> GGTAYWKNPDQFTAFNTGLHALLREKSYNFFLLGEPRADIYGDNPIGGEASQGMERLPFNTINKENVGISNYGDMYKIINQINQMIAKTTETTILTEATQNYYLGEAYGMRAYLYFHLLRSWGDVVLYLDY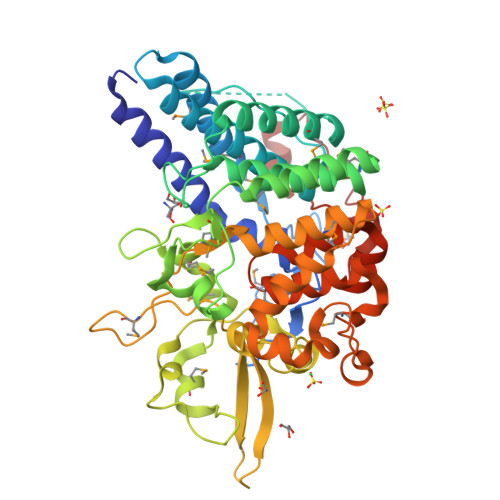TEGQNLDLSNITKGVSPATEVMEQIKKDIQASENAFGSDYSFKLGRHFWSAAATQMLKGEAYLWSGRQMNGGNSDYTIAKNAFENVKKADVGLVTSSFKDIFSFENKKNKEMIFTIHNGKDEYEMWGGYYRMRLIPAQDKMVKIYCDENGNSFVGTPDAQLNGLTQLQVRREFYFKGFRNNDTRWTTSLKAVYKKDAQGVVSYFGPITYKFQGTMLEGGSTRSFLDDFPIYRYADCLLQLAMAKVLLGEDPTEEINAVRERAYGSKYFNEHKAEIAYPNDNDPEFYTDNKWMKPDNAGALEAILKERLREFMFEGKRWYDIRLLGWDYVHQYSSAEQSRLLWPIDAGTLTNNSALKQTPGYE Cohesin is loaded onto chromatin by the Scc2-Scc4 loader complex, however persistent cohesion cannot be established without the acetylation of two conserved tandem lysines on the Smc3 subunit by the Eco1 acetyltransferase (ACT). Eco1 is an acetyltransferase that belongs to the Gcn5-related N-acetyltransferase (GNAT) family. The xEco2 ACT fold is divided into two domains: the N-terminal domain contains α helix 1 and 2, and β strand 1–5 with a conserved central β hairpin insertion between β4 and β5 that is unique to cohesin ACTs; the C-terminal domain contains α helix 3, and β strand 6 and 7. The binding site for CoA is sandwiched between the N- and C-terminal domains involving β5 and α3, while the substrate peptides binds mainly to the central β hairpin and the C-terminal domain including the conserved C-terminal extension (C extension).

To gain insights into Smc3 recognition by Eco1, we performed crystallographic studies on the Xenopus laevis Eco2 (xEco2) ACT domain (residues 523–702), with and without the binding to its canonical Smc3 substrate peptides. Crystals of the peptide-free xEco2 (henceforth xEco2) diffracted to 3.0 Å, whereas the binding of the K105-CoA and K106-CoA peptides to xEco2 improved the resolution to 2.4 and 1.9 Å respectively. In the peptide-free xEco2 structure, the conserved W623 occupying the hydrophobic pocket is partially stacked against the conserved F700 on the C extension. However, this mode of dimerization was not observed in either our peptide-free or substrate-bound crystal forms. To define the oligomeric state of xEco2, we performed multi-angle light scattering (MALS) and determined the solution masses of the free and substrate-bound ACT domain to be 25.5 and 26.7 (+/−0.54) kDa respectively, indicating their monomeric states in our system. The peptide-free form of xEco2 crystallized in 0.2 M NaCl, 0.1 M imidazole pH 7 and 0.864 M ammonium phosphate. The peptide-free and K105-CoA structures were solved using the K106-CoA structure as a start model in Phaser and multiple rounds of re-building and refinement were carried out as described.

>GSMKKERVITEFWDGKIIMVSPDDPKYALKKAEEVRELVDSELGFQQVSLRCPSQTRTYMFVSNEKKIVGCLIAEPIREAYRVLAEPPSLHSLHGEPLERHRAWRCSTEPEPAICGISRIWVFALMRRKAIASRMVDAVRSSFMYGSVLTTEEIAFSDPTPDGKLFASTYCKVPDFLVYNFVS[2x]>[4x]HHHHHHVPAFLTKLWTLVSDPDTDALICWSPS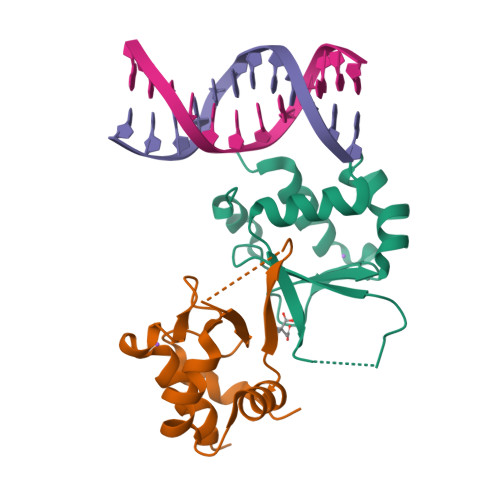GNSFHVFDQGQFAKEVLPKYFKHNNMASFVRQLNMYGFRKVVHIEQGGLVKPERDDTEFQHPCFLRGQEQLLENIKRKVT> SLNPGVDAMYCKQWPE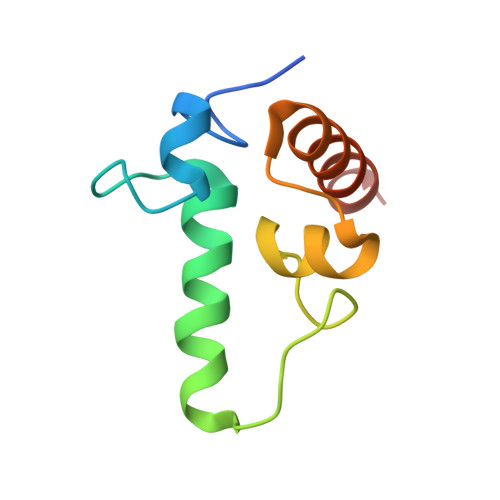CAKKMSANCICLLCLLRMKHENRKLYRKDPLVWVDCYCFDCFRMWFGLDLCEGTLLLWCDIIGQTTYRDLKL>[10x]MTIKYLSSETEKLMNQTVSGIDVCFTLIGVDDDSFASGSKNDYISDTPKFLDPSNVHIKATLKRGGKDYVLFSENLALLAKYSTITQGRDQWEEGVKLAAKEMVHLVYIPFSGNTNWPAHINLKDNDVLEVYVNVVRGAYGAELDANACICDVRTSPSIGVEKFIPFMTSYSIRANQATDLVNLGNDVTRIALLSMTNDVSNIPNAFTDVTLSSDRLDKNFNSN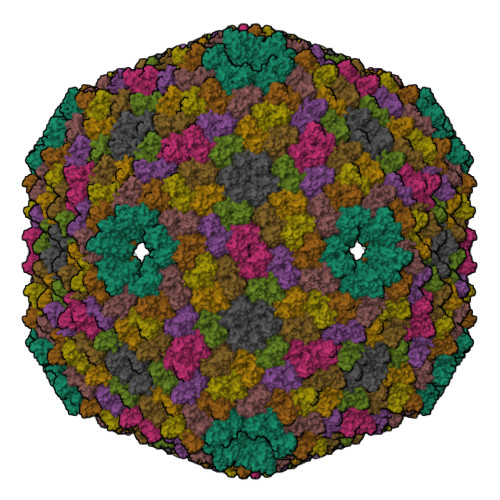QLILEHSKCIEDSVRSHANEVDSYLIHEDIEIDSAKVHLKMNPAKIRENTIYLVRSHFQTSLEILQKAVAMEEKHQSADIAKVPAT> MPFVNKQFNYKDPVNGVDIAYIKIPNAGQMQPVKAFKIHNKIWVIPERDTFTNPEEGDLNPPPEAKQVPVSYYDSTYLSTDNEKDNYLKGVTKLFERIYSTDLGRMLLTSIVRGIPFWGGSTIDTELKVIDTNCINVIQPDGSYRSEELNLVIIGPSADIIQFECKSFGHEVLNLTRNGYGSTQYIRFSPDFTFGFEESLEVDTNPLLGAGKFATDPAVTLAHELIHAGHRLYGIAINPNRVFKVNTNAYYEMSGLEVSFEELRTFGGHDAKFIDSLQENEFRLYYYNKFKDIASTLNKAKSIVGTTASLQYMKNVFKEKYLLSEDTSGKFSVDKLKFDKLYKMLTEIYTEDNFVKFFKVLNRKTYL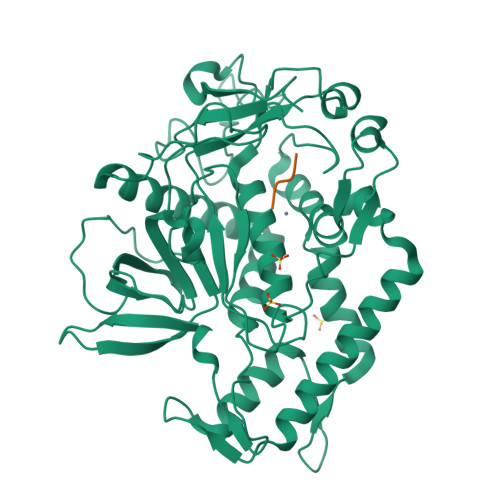NFDKAVFKINIVPKVNYTIYDGFNLRNTNLAANFNGQNTEINNMNFTKLKNFTGLFELEHHHHHH;> RRGIX> MKLERVTVKNFRSHSDTVVEFKEGINLIIGQNGSGKSSLLDAILVGLYWPLRIKDIKKDEFTKVGARDTYIDLIFEKDGTKYRITRRFLKGYSSGEIHAMKRLVGNEWKHVTEPSSKAISAFMEKLIPYNIFLNA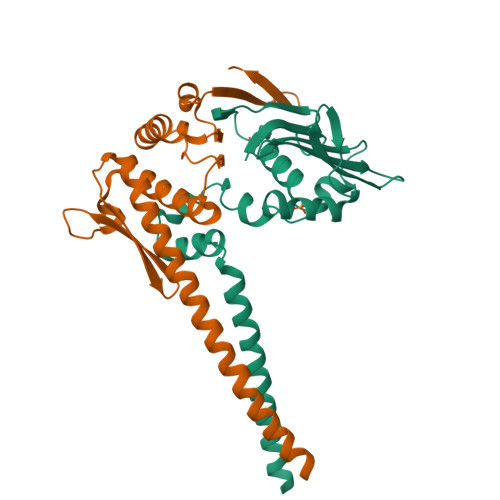IYIRQGQIDAILESDEAREKVVREVLNLDKFETAYKKLSELKKTINNRIKEYRDILARTE;> RERVKKEIKDLEKAKDFTEELIEKVKKYKALAREAALSKIGELASEIFAEFTEGKYSEVVVRAEENKVRLFVVWEGKERPLTFLSGGERIALGLAFRLAMSLYLAGEISLLILDEPTPYLDEERRRKLITIMERYLKKIPQVILVSHDEELKDAADHVIRISLENGSSKVEVVS> MEPSQCVEELEDD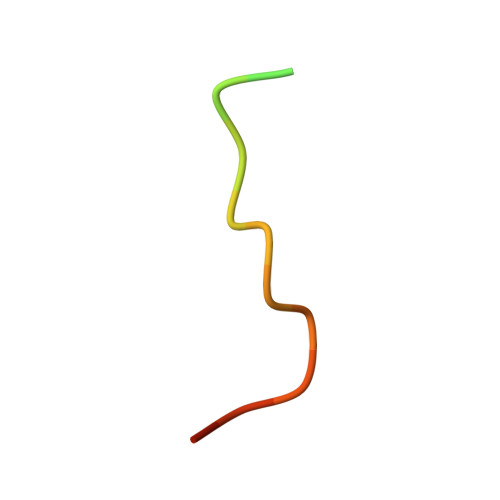VFQPED>GVKIMPNLPGLYFLQAYPSEEIWRLFVDGRFWSKENGWRGYESREPGCLNAALESLCSIALQVEKSGEEFELSVDLIKRIHKKCGKKVEELQEKNPGELRTDEPVSFGIPAGRASIKGIEEFLSLVFLTEGGAEFGPGKAGPFGPRFDKNYFKNLNPEQIPDLAKQIYFDMCKYGHSNTNHFYLAVMKNVDVYLEKITQSYNKEIKTAETLDEKLKIIVKHIRMYEVLHPFRDANGRTFVNNLLNIPLMQQGLPPATFYEPNVFDLYSAEELVVVVKEAIFNTVEIIEQSKRKTPITLYGYHSSLEEQTKFRDMLDSPSYEKIKHMDFSDLNPEKLHLKTQKCLSSLNEQYPLHRGAIYLSDPGEIKLLLSNRNESQINQQIEQGAPPIYVGKTPAHLAVISGNMAMLDELIAKKADLSLQDYDGKTALHYAAECGNMQI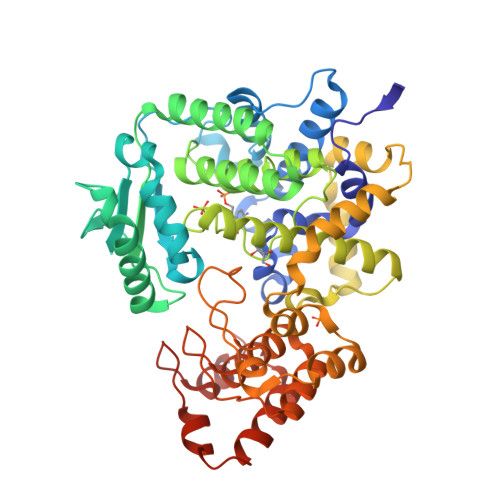MGKILKVVLSQEDAIKVLNIKDNHGKTAFHYAAEFGTPELISAL[2x]> MKSVVTTVLAAADAAGRFP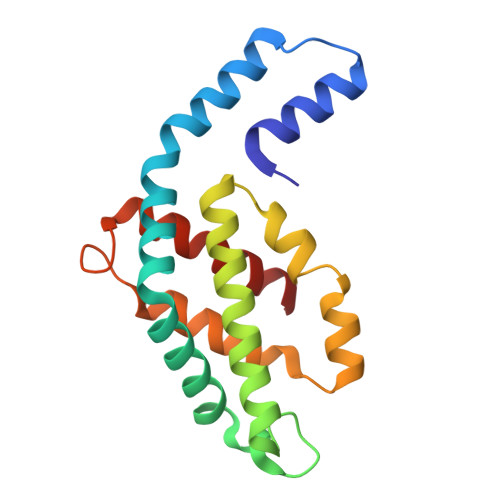SGSDLESVQGNIQRSAARLEAAEKLAAGHAAVVKEAGDVVFKKYPYLKTAGEAGDSAEKVAKCYRDIDHYMRLINYCLVVGGTGPLDEWGISGAREVYRALNLPTAAYVAAFQYTRDRACAPRDMGPQALTEFRSYLDYVINALS> MLHLSAAPPAPPPEVTATARPCLCSVGRRGDGGKMAAAGALERSFVELSGAERERPRHFREFTVCSIGTANAVAGAVKYSESAGGFYYVESGKLFSVTRNRFIHWKTSGDTLELMEESLDINLLNNAIRLKFQNCSVLPGGVYVSETQNRVIILMLTNQTVHRLLLPHPSRMYRSELVVDSQMQSIFTDIGKVDFTDPCNYQLIPAVPGISPNSTASTAWLSSDGEALFALPCASGGIFVLKLPPYDIPGMVSVVELKQSSVMQRLLTGWMPTAIRGDQSPSDRPLSLAVHCVEHDAFIFALCQDHKLRMWSYKEQMCLMVADMLEYVPVKKDLRLTAGTGHKLRLAYSPTMGLYLGIYMHAPKRGQFCIFQLVSTESNRYSLDHISSLFTSQETLIDFALTSTDIWALWHDAENQTVVKYINFEHNVAGQWNPVFMQPLPEEEIVIRDDQDPREMYLQSLFTPGQFTNEALCKALQIFCRGTERNLDLSWSELKKEVTLAVENELQGSVTEYEFSQEEFRNLQQEFWCKFYACCLQYQEALSHPLALHLNPHTNMVCLLKKGYLSFLIPSSLVDHLYLLPYENLLTEDETTISDDVDIARDVICLIKCLRLIEESVTVDMSVIMEMSCYNLQSPEKAAEQILEDMITIDVENVMEDICSKLQEIRNPIHAIGLLIREMDYETEVEMEKGFNPAQPLNIRMNLTQLYGSNTAGYIVCRGVHKIASTRFLICRDLLILQQLLMRLGDAVIWGTGQLFQAQQDLLHRTAPLLLSYYLIKWGSECLATDVPLDTLESNLQHLSVLELTDSGALMANRFVSSPQTIVELFFQEVARKHIISHLFSQPKAPLSQTGLNWPEMITAITSYLLQLLWPSNPGCLFLECLMGNCQYVQLQDYIQLLHPWCQVNVGSCRFMLGRCYLVTGEGQKALECFCQAASEVGKEEFLDRLIRSEDGEIVSTPRLQYYDKVLRLLDVIGLPELVIQLATSAITEAGDDWKSQATLRTCIFKHHLDLGHNSQAYEALTQIPDSSRQLDCLRQLVVVLCERSQLQDLVEFPYVNLHNEVVGIIESRARAVDLMTHNYYELLYAFHIYRHNYRKAGTVMFEY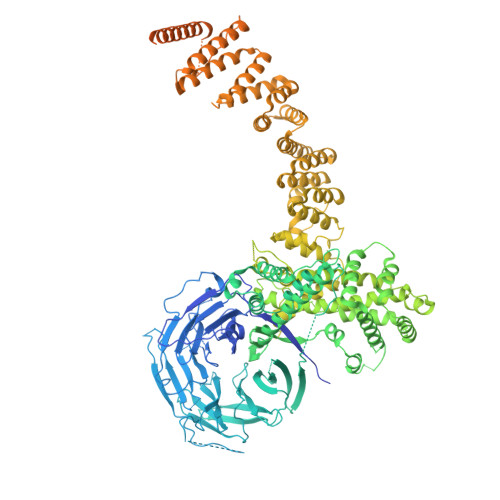GMRLGREVRTLRGLEKQGNCYLAALNCLRLIRPEYAWIVQPVSGAVYDRPGASPKRNHDGECTAAPTNRQIEILELEDLEKECSLARIRLTLAQHDPSAVAVAGSSSAEEMVTLLVQAGLFDTAISLCQTFKLPLTPVFEGLAFKCIKLQFGGEAAQAEAWAWLAANQLSSVITTKESSATDEAWRLLSTYLERYKVQNNLYHHCVINKLLSHGVPLPNWLINSYKKVDAAELLRLYLNYDLLEEAVDLVSEYVDAVLGKGHQYFGIEFPLSATAPMVWLPYSSIDQLLQALGENSANSHNIALSQKILDKLEDYQQKVDKATRDLLYRRTL>[2x]GSRTVDLELELQIELLRETKRKYESVL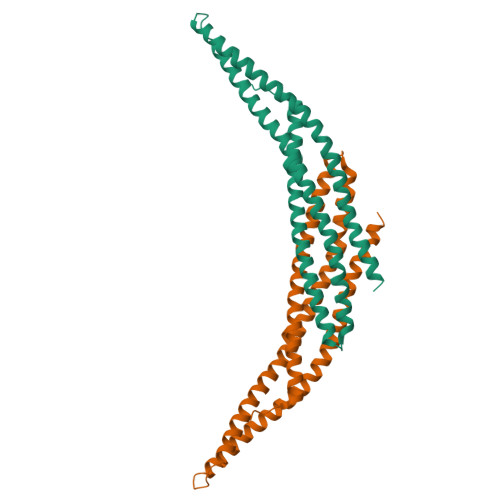QLGRALTAHLYSLLQTQHALGDAFADLSQKSPELQEEFGYNAETQKLLCKNGETLLGAVNFFVSSINTLVTKTMEDTLMTVKQYEAARLEYDAYRTDLEELSLGPRDAGTRGRLESAQATFQAHRDKYEKLRGDVAIKLKFLEENKIKVMHKQLLLFHNAVSAYFAGNQKQLEQTLQQFNIKLRPPGAEKPSWLEEQ>MAPKAVLVGLPGSGKSTIGRRLAKALGVGLLDTDVAIEQRTGRSIADIFA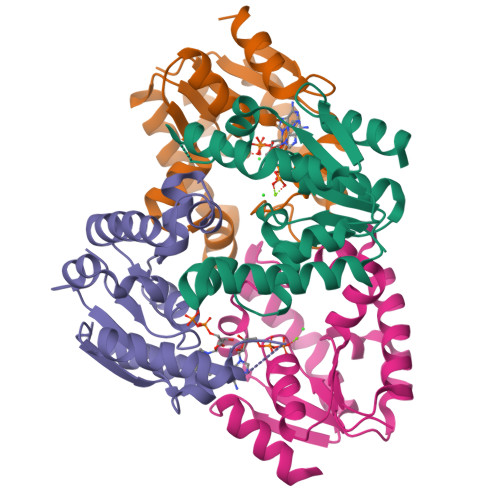TDGEQEFRRIEEDVVRAALADHDGVLSLGGGAVTSPGVRAALAGHTVVYLEISAAEGVRRTGGNTVRPLLAGPDRAEKYRALMAKRAPLYRRVATMRVDTNRRNPGAVVRHILSRLQVPSPSEAAT[4x]> MAEPVSPLKHFVLAKKAITAIFDQLLEFVTEGSHFVEATYKNPELDRIATEDDLVEMQGYKDKLSIIGEVLSRRHMKVAFFGRTSSGKSSVINAMLWDKVLPSGIGHITNCFLSVEGTDGDKAY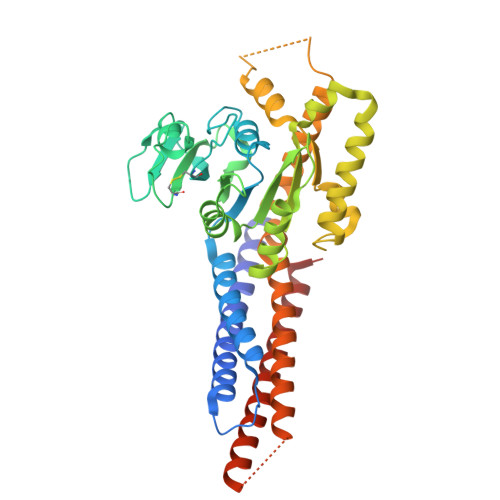LMTEGSDEKKSVKVNNQLAHALHMDKDLKAGCLVRVFWPKAKCALLRDDLVLVDSPGTDVTTELDSWIDKFCLDADVFVLVANSESTLMNTEKHFFHKVNERLSKPNIFILNNRWDASASEPEYMEDVRRQHMERCLHFLVEELKVVNALEAQNRIFFVSAKEVLSARKQKAQGMPESGVALAEGFHARLQEFQNFEQIFEECISQSAVKTKFEQHTIRAKQILATVKNIMDSVNLAAEDGSGSGSGGSEIARLPKEIDQLEKIQNNSKLLRNKAVQLENELENFTKQFLPSSNEES>[3x]MSTVGTGKLTRAQRRAAARKNKRNTRVVQPVIVEPIASGQGKAIKAWTGYSVSKWTASCAAAEAKVTSAITISLPNELSSERNKQLKVGRVLLWLGLLPSVSGTVKSCVTETQTTAAASFQVALAVADNSKDVVAAMYPEAFKGITLEQLTADLTIYLYSSAALTEGDVIVHLEVEHVRPTFDDSFTPVY

Cowpea chlorotic mottle virus is an icosahedrally symmetric plant virus in the Bromoviridae family that infects cowpea plants (Vigna unguiculata). The 180 identical capsid proteins are arranged in 12 pentamers and 20 hexamers. The asymmetric unit (highlighted) contains three subunits A, B, and C (magenta, green, and blue, respectively). CCMV is thought to achieve this by detecting a change in its chemical environment upon entering the host cell, which causes its capsid to swell, increasing in diameter by about 10%2.

Once the calcium ions are no longer present to compensate these negative charges, electrostatic repulsion causes the capsid to expand. In the absence of divalent ions, the virus can also be artificially contracted by lowering the pH below 5, which protonates the negatively charged residues and thus removes their repulsion. In contrast, a sample prepared at pH 5.0 yields the structure of the fully contracted state with a diameter of 28 nm. The resolution of 1.6 Å is considerably higher than that of the extended state, which is more flexible and prone to partial disassembly. We then dock atomic models of the extended configuration into slices 1–12 (extended and partially contracted particles) and of the contracted configuration into slices 25–30 (fully contracted particles), from which we determine the motions of the capsid proteins. The contraction of CCMV is accompanied by a simultaneous anticlockwise rotation of the pentamers and hexamers, which are both rotated by about 5 degrees in the fully contracted state. It reveals that the pentamers rotate about twice as fast as the hexamers, adopting a rotation angle of over 3 degrees in slice 12, while the hexamers reach only about 1.5 degrees. This rotation of the capsomeres is accompanied by a superimposed rotation of the capsid subunits around the axes indicated with black arrows in Fig. 4a. However, whereas subunit A has already reached its final rotation angle of ~7 degrees in slice 12, subunits B and C have completed only about half their rotations of ~11 and ~13 degrees, respectively. The process thus resembles a collapse that is triggered when the electrostatic repulsion is removed that keeps the capsid inflated.3-chloro-2-hydroxy-N-{2-[(4-methyl-4H-1,2,4-triazol-3-yl)sulfanyl]phenyl}benzene-1-sulfonamide 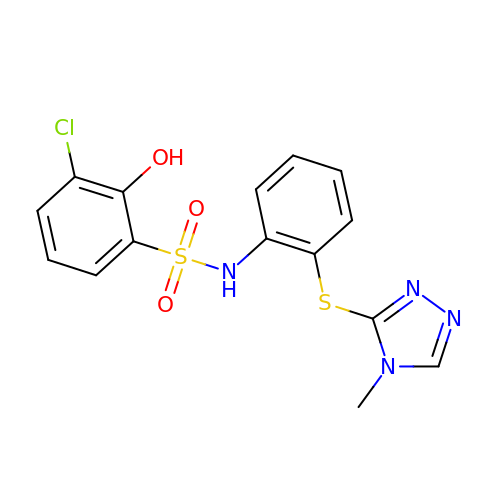| C15 H13 Cl N4 O3 S2 | DNTLDOPFKLUBET-UHFFFAOYSA-N> AWITAPVALREGEDLSKKNPIAKIHSDLAEERGLKITYKYTGKGITEPPFGIFVFNKDTGELNVTSILDREETPFFLLTGYALDARGNNVEKPLELRIKVLDINDNEPVFTQDVFVGSVEELSAAHTLVMKINATDADEPNTLNSKISYRIVSLEPAYPPVFYLNKDTGEIYTTSVTLDREEHSSYTLTVEARDGNGEVTDKPVKQA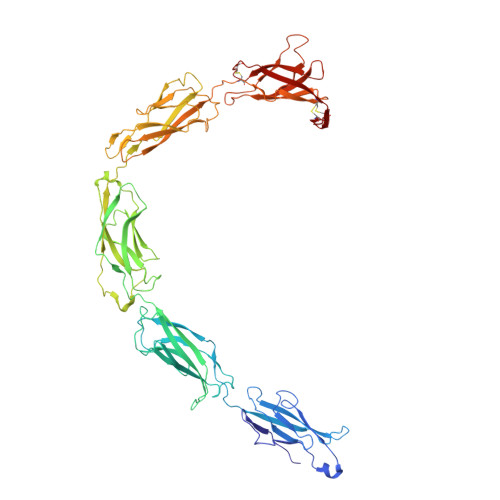QVQIRILDVNDNIPVVENKVLEGMVEENQVNVEVTRIKVFDADEIGSDNWLANFTFASGNEGGYFHIETDAQTNEGIVTLIKEVDYEEMKNLDFSVIVANKAAFHKSIRSKYKPTPIPIKVKVKNVKEGIHFKSSVISIYVSESMDRSSKGQIIGNFQAFDEDTGLPAHARYVKLEDRDNWISVDSVTSEIKLAKLPDFESRYVQNGTYTVKIVAISEDYPRKTITGTVLINVEDINDNCPTLIEPVQTICHDAEYVNVTAEDLDGHPNSGPFSFSVIDKPPGMAEKWKIARQESTSVLLQQSEKKLGRSEIQFLISDNQGFSCPEKQVLTLTVCECLHGSGCREAH>SSVPLEWPLSSQSGSYELRIEVQPKPHHRAHYETEGSRGAVKAPTGGH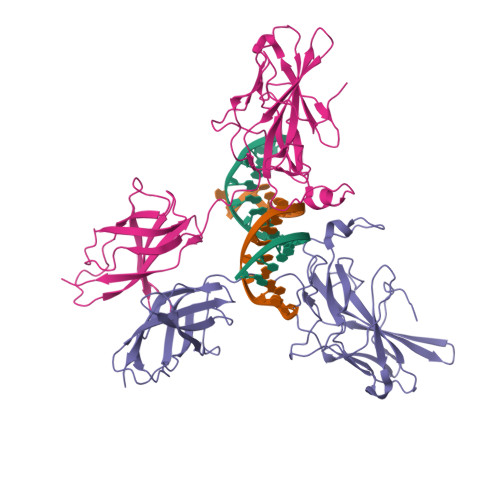PVVQLHGYMENKPLGLQIFIGTADERILKPHAFYQVHRITGKTVTTTSYEKIVGNTKVLEIPLEPKNNMRATIDCAGILKLRNADIELRKGETDIGRKNTRVRLVFRVHIPESSGRIVSLQTASNPIECSQRSAHELPMVERQDTDSCLVYGGQQMILTGQNFTSESKVVFTEKTTDGQQIWEMEATVDKDKSQPNMLFVEIPEYRNKHIRTPVKVNFYVINGKRKRSQPQHFTYHPV[4x]>[2x]MDDANKIRREEVLVSMCDQRARMLQDQFSVSVNHVHALAILVSTFHYHKNPSAIDQETFAEYTARTAFERPLLSGVAYAEKVVNFEREMFERQHNWVIKTMDRGEPSPVRDEYAPVIFSQDSVSYLESLDMMSGEEDRENILRARETGKAVLTSPFRLLETHHLGV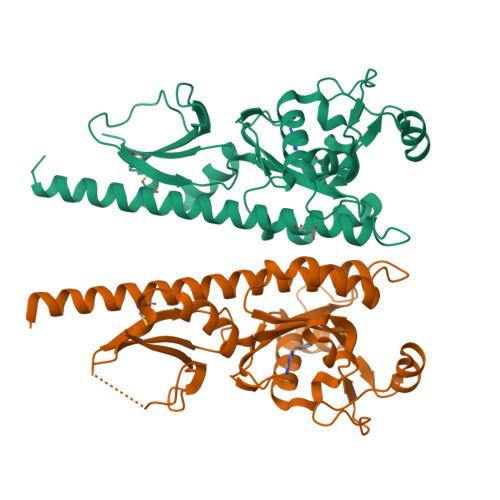VLTFPVYKSSLPENPTVEERIAATAGYLGGAFDVESLVENLLGQLAGNQAIVVHVYDITNASDPLVMYGNQDEEADRSLSHESKLDFGDPFRKHKMICRYHQKA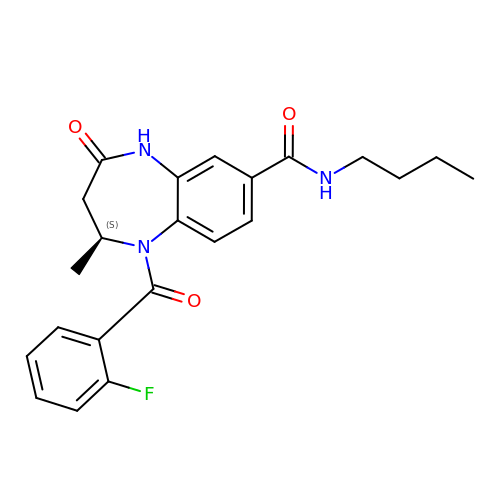(2S)-N-butyl-1-(2-fluorophenyl)carbonyl-2-methyl-4-oxidanylidene-3,5-dihydro-2H-1,5-benzodiazepine-7-carboxamide | C22 H24 F N3 O3 | RZHHEEJRHNWMHI-AWEZNQCLSA-N> MDVVSLDKPFMYFEEIDNELDYEPESANEVAKKLPYQGQLKLLLGELFFLSKLQRHGILDGATVVYIGSAPGTHIRYLRDHFYNLGVIIKWMLIDGRHHDPILNGLRDVTLVTRFVDEEYLRSIKKQLHPSKIILISDVRSKRGGNEPSTADLLSNYALQNVMISILNPVASSLKWRCPFPDQWIKDFYIPHGNKMLQPFAPSYSAEMRLLSIYTGENMRLTRVTKSDAVNYA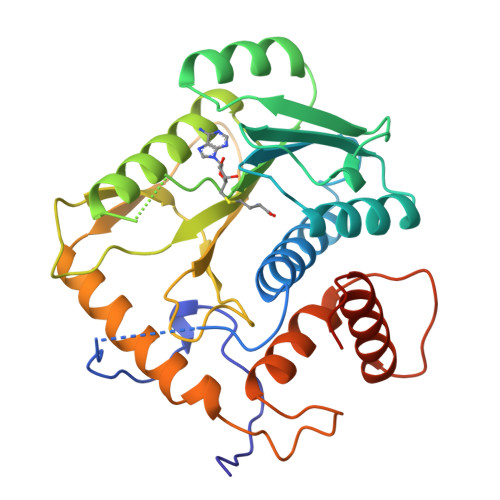KKMYYLNKIVRNKVVVNFDYPNQEYDYFHMYFMLRTVYCNKTFPTTKAKVLFLQQSIFRFLNIPTTSTEKVSHE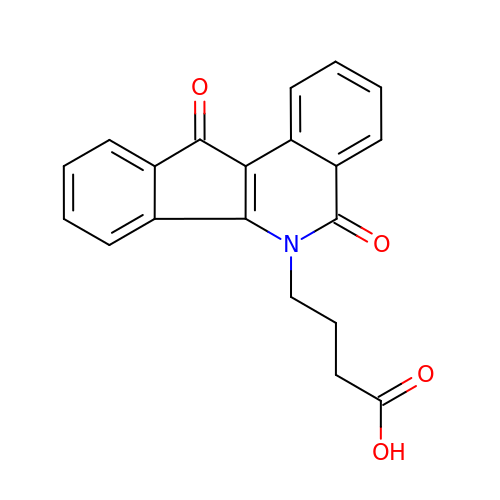4-(5,11-DIOXO-5H-INDENO[1,2-C]ISOQUINOLIN-6(11H)-YL)BUTANOATE | C20 H15 N O4 | AHIJTWCJGCWHMT-UHFFFAOYSA-N> GEFMEEGKMDENEWSYHGEGNKSLVVAHAQRCVVLRFLKFPPNKKKTSEEILQHLQNIVDFGKNVMKDFLGENYVHCGEVV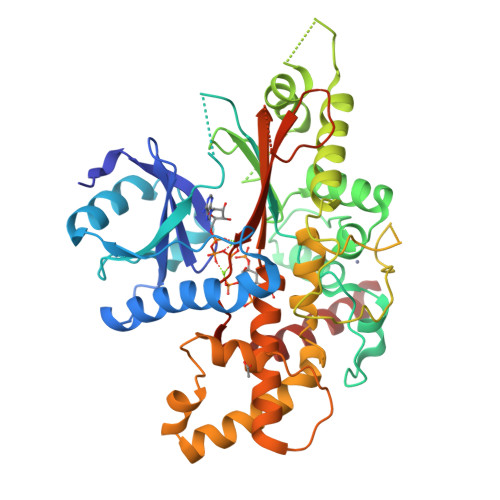QLPLEFVKQLCLKIQCERPESRCDKDLDTFSGYAMCLPNLTRLQTFHFAEHRPILCVEIKPKCGFIPFSNDVTHEMKHKVCRYCMHQHLKVATGKWKKISKYCPLDLYSGNKQRMHFALRSLLQETQNNLRIFKNGELIYGCGDARSPVADLKELAHHLKPFFFPSNGLASGPHCTKAVIRELVHVITRVLLSSSEKARAGALRLGLQGPRVCEASPFSRSLHNQGKNTSEHSGLPKGCLLYKTLQVQMLDQLDIEGLYPLYKRVEQYLEEFPEERKTLQIDGPYDEVFYQKLLDLSTEDDGTVAFALTKVQQYRVAMTAKDCSIMIALSPCLQGTSSDQRPVIPSSRSRLAFSVSVLDLDLKPYESIPHQYKLDSKIVNYYSKTVHAKD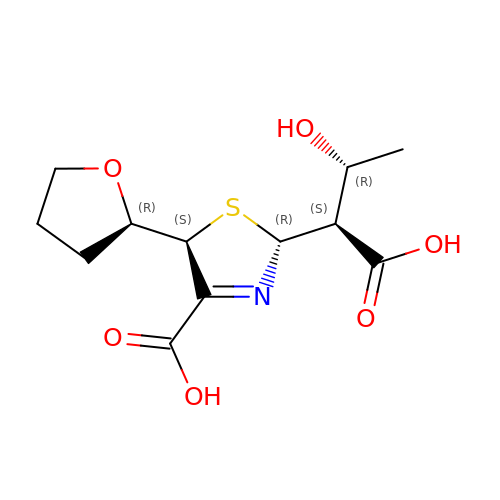(2R,5S)-2-[(1S,2R)-1-carboxy-2-hydroxy-propyl]-5-[(2R)-tetrahydrofuran-2-yl]-2,5-dihydrothiazole-4-carboxylic acid | C12 H17 N O6 S | SVIXNOHLIBGRQI-CTNSIQBBSA-N>[2x]MAAHLSYGRVNLNVLREAVRRELREFLDKCAGSKAIVWDEYLTGPFGLIAQYSLLKEHEVEKMFTLKGNRLPAADVKNIIFFVRPRLELMDIIAENVLSEDRRGPTRDFHILFVPRRSLLCEQRLKDLGVLGSFIHREEYSLDLIPFDGDLLSMESEGAFKECYLEGDQTSLYHAAKGLMTLQALYGTIPQIFGKGECARQVANMMIRMKREFTGSQNSIFPVFDNLLLLDRNVDLLTPLATQLTYEGLIDEIYGIQNSYVKLPPEKFAPKKQGDGGKDLPTEAKKLQLNSAEELYAEIRDKNFNA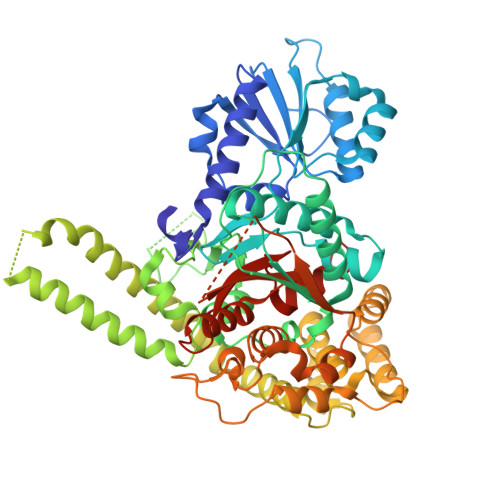VGSVLSKKAKIISAAFEERHNAKTVGEIKQFVSQLPHMQAARGSLANHTSIAELIKDVTTSEDFFDKLTVEQEFMSGIDTDKVNNYIEDCIAQKHSLIKVLRLVCLQSVCNSGLKQKVLDYYKREILQTYGYEHILTLHNLEKAGLLKPQTGGRNNYPTIRKTLRLWMDDVNEQNPTDISYVYSGYAPLSVRLAQLLSRPGWRSIEEVLRILPGPHFEERQPLPTGLQKKRQPGENRVTLIFFLGGVTFAEIAALRFLSQLEDGGTEYVIATTKLMNGTSWIEALMEKPFHHHHHHHHHHH>[2x]LPKKRYYRQRAHSNPFSDHQLEYPVSPQDMDWSKLYPYYKNAENGQMTKKVTIADIGCGFGGLMIDLSPAFPEDLILGMEIRVQVTNYVEDRIIALRNNT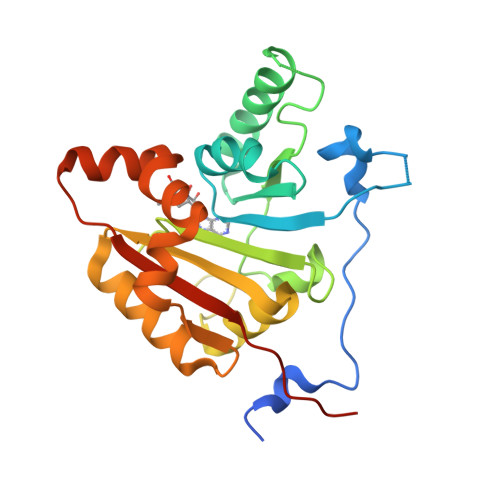ASKHGFQNINVLRGNAMKFLPNFFEKGQLSKMFFCFPDPHFKQRKHKARIITNTLLSEYAYVLKEGGVVYTITDVKDLHEWMVKHLEEHPLFERLSKEWEENDECVKIMRNATEEGKKVERKKGDKFVACFTRLPTPAILHHHHHH>[3x]NRILPDSVDWREKGCVTEVKYQGSCGACWAFSAVGALEAQLKLKTGKLVSLSAQNLVDCSTEKYGNKGCNGGFMTTAFQYIIDNKGIDSDASYPYKAMDQKCQYDSKYRAA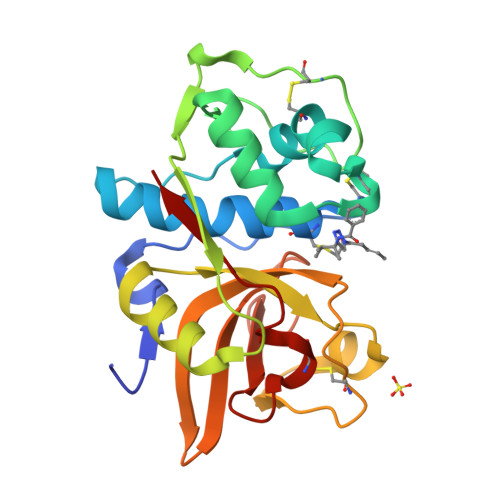TCSKYTELPYGREDVLKEAVANKGPVSVGVDARHPSFFLYRSGVYYEPSCTQNVNHGVLVVGYGDLNGKEYWLVKNSWGHNFGEEGYIRMARNKGNHCGIASFPSYPEI>MLPAPKNLVVSEVTEDSARLSWDDPAAFYESFLIQYQESEKVGEAIVLTVPGSERSYDLTGLKPGTEYTVSIYGV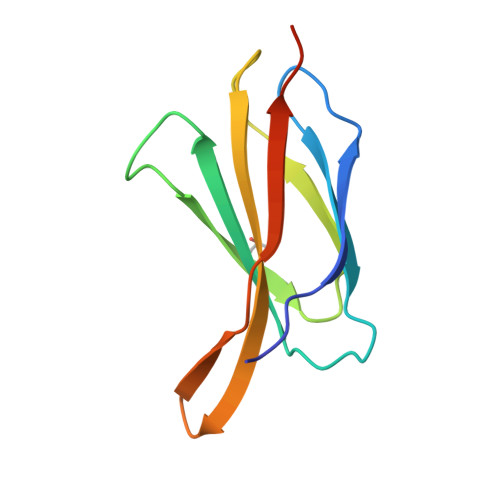HNVYKDTNMRGLPLSAIFTTGGHHHHHH[4x]>MNPIVINRLQRKLGYTFNHQELLQQALTHRSASSKHNARLEFLGDSILSYVIANALYHRFPRVDAGDMSRMRATLVRGNTLAELAREFELGECLRLGPGELKSGGFRRESILADTVEALIGGVFLDSDIQTVEKLILNWYQTRLDEISPGDKQKDPKTRLQEYLAGRHLPLPTYLVVQVRGEAHDQEFTIHCQVSGLSEPVVGTGSSRRKAEQAAAEQALKKLELE[2x]

Discovered in 1968, Escherichia coli RNase III (EcRNase III) is the founding member of the RNase III family of dsRNA-specific endoribonucleases found in all kingdoms of life. Among the four representative family members, Rnt1p and Drosha process stem-loop RNAs only, whereas RNase III and Dicer also process long dsRNAs. Bacterial RNase III functions as a dimer, and thus removing two negatively charged side chains between the protein and RNA promotes consecutive binding and cleavage of long dsRNA by multiple RNase III dimers. Each EcEEQ molecule contains a specialized endonuclease domain (RIIID, residues 1–147) and a dsRNA-binding domain (dsRBD, residues 156–226).

Here, we report the crystal structure of EcEEQ in complex with a stem-loop RNA (RNA6) at 1.80-Å resolution (EcEEQ:RNA6), showing how the E38A and E65A mutations stabilize the protein:RNA complex and how the Q165A mutation eliminates the sequence specificity of EcRNase III. The complex is composed of two EcEEQ subunits (each containing 226 amino acid residues), two RNA6 molecules (each containing 28 nucleotide residues in the form of a hairpin with a 4-nucleotide capping loop and a 2-nucleotide 3ʹ overhang), six Mg2+ ions, 418 water oxygen atoms, and several other ions and molecules from the solvent and cryoprotectant. Hence, the EcEEQ:RNA6 structure resembles the postcleavage complex of AaRNase III, indicating that the EcEEQ:RNA6 complex is also a postcleavage complex. Therefore, the alanine mutation of both E38 and E65 stabilizes the resulting protein:RNA complex and thereby promotes the inside-out processing of long dsRNAs. Hence, the Q165A mutation eliminates these strong hydrogen bonds and thereby abolishes its specificity for the +3 G nt. In each cleavage site of the EcEEQ:RNA6 structure, three Mg2+ ions are well defined and fully occupied. As depicted in Figure 4(a), these Mg2+ ions (MgA, MgB and MgC) are ‘organizers’ of the cleavage site assembly by coordinating with four catalytic side chains (E41, D45, D114, and E117), three nucleotide residues (R-1, R 0, and R+1), and eight water molecules around the scissile bond. The CDMgA,MgB in the EcEEQ:RNA6 structure is 3.7 Å, suggesting that the EcEEQ:RNA6 structure represents the postcleavage state immediately after the intermediate state of RNA hydrolysis. It appears that MgC plays three important roles in catalysis. We predict that all prokaryotic RNase IIIs employ the third Mg2+ ion to assist two-Mg2+-ion catalysis of RNA hydrolysis.>[4x]GSSETQRQFSRYFIEFEELQLLGKGAFGAV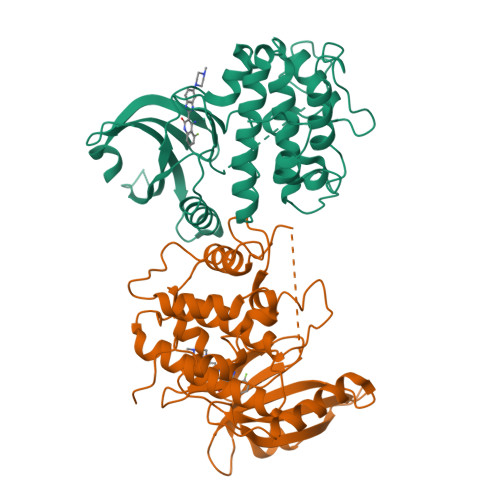IKVQNKLDGCCYAVKRIPINPASRQFRRIKGEVTLLSRLHHENIVRYYNAWIERHERPSVTTEAVHYLYIQMEYCEKSTLRDTIDQGLYRDTVRLWRLFREILDGLAYIHEKGMIHRNLKPVNIFLDSDDHVKIGDFGLATDHLAFSADSKQDDQTGDLIKSDPSGHLTGMVGTALYVSPEVQGSTKSAYNQKVDLFSLGIIFFEMSYHPMVTASERIFVLNQLRDPTSPKFPEDFDDGEHAKQKSVISWLLNHDPAKRPTATELLKSELLPPPQMEESELHEVLHHTLT N-{(2S)-4-(methylamino)-4-oxo-2-[4-(phosphonooxy)benzyl]butanoyl}-L-isoleucyl-L-aspartamide 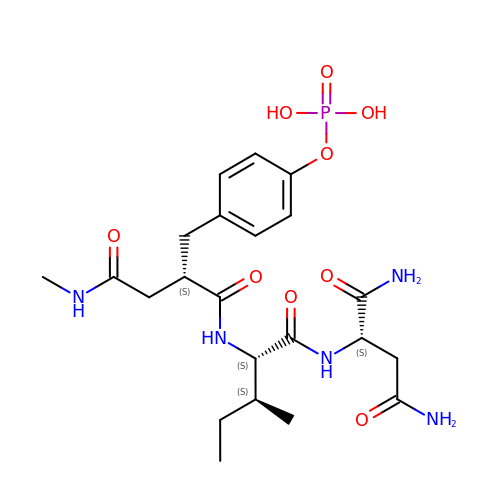| C22 H34 N5 O9 P | UEYBGJJDTRNDGF-HAHWVIBASA-N>MAKHVVVIGGGVGGIATAYNLRNLMPDLKITLISDRPYFGFTPAFPHLAMGWRKFEDISVPLAPLLPKFNIEFINEKAESIDPDANTVTTQSGKKIEYDYLVIATGPKLVFGAEGQEENSTSICTAEHALETQKKLQELYANPGPVVIGAIPGVSCFGPAYEFALMLHYELKKRGIRYKVPMTFITSEPYLGHFGVGGIGASKRLVEDLFAERNIDWIANVAVKAIEPDKVIYEDLNGNTHEVPAKFTMFMPSFQGPEVVASAGDKVANPANKMVIVNRCFQNPTYKNIFGVGVVTAIPPIEKTPIPTGVPKTGMMIEQMAMAVAHNIVNDIRNNPDKYAPRLSAICIADFGEDAGFFFADPVI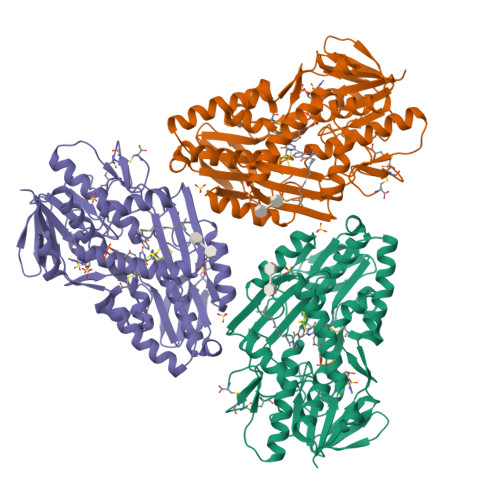PPRERVITKMGKWAHYFKTAFEKYFLWKVRNGNIAPSFEEKVLEIFLKVHPIELCKDCEGAPGSRC[6x]> ISGGDAIYSSTGRCSLGFNVRSGSTYYFLTAGHCTDGA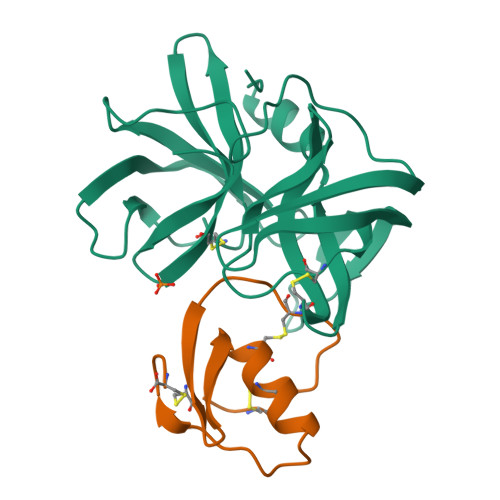TTWWANSARTTVLGTTSGSSFPNNDYGIVRYTNTTIPKDGTVGGQDITSAANATVGMAVTRRGSTTGTHSGSVTALNATVNYGGGDVVYGMIRTNVCAEPGDSGGPLYSGTRAIGLTSGGSGNCSSGGTTFFQPVTEALVAYGVSVY;> VDCSEYPKPACTAEYRPLCGSDNKTYGNKCNFCNAVVESNGTLTLSHFGKC FMS-like tyrosine kinase 3 (FLT3) is a receptor tyrosine kinase that is expressed in both normal and malignant lympho-hematopoietic cells and is important for immune response and stem cell proliferation. The characteristic domain organization of these receptors includes an extracellular module, a transmembrane (TM) helix, and an intracellular module that consists of a juxtamembrane (JM) segment, a kinase domain with a kinase insert region, and a C-terminal tail. The deregulated activation of FLT3 due to mutation or overexpression is linked to the progression of acute myeloid leukemia (AML) and is associated with poor prognosis. Chemical optimization of these compounds led to the discovery of quizartinib or AC220, which exhibits both selectivity for and potency against FLT3.

Here, we determined the co-crystal structure of FLT3 bound to quizartinib. FLT3 adopts an “Abl-like” inactive conformation with quizartinib bound. The DFG motif adopts a “DFG-out” conformation, the activation loop is folded back onto the kinase domain to mimic peptide substrate binding, and Glu 661 on the αC helix forms a salt bridge with Lys 644 in the active site. One favorable interaction observed in the quizartinib-FLT3 co-crystal structure, in contrast to the top-ranked docking pose, is between the tert-butyl substituent on the isoxazole ring of quizartinib and a hydrophobic pocket on FLT3. The pocket includes Met 664 and Met 665 on the αC helix, Ile 674 in the N lobe, Leu 802 in the C lobe, and Ile 827, which is immediately N terminal to the DFG motif. The carbonyl group of the urea forms hydrogen bond interactions with the backbone nitrogen of Cys 828. Further, the nitrogens in the urea moiety form hydrogen bond interactions with Glu 661 in the αC helix. The central para-substituted phenyl ring on quizartinib makes key interactions in the kinase active site of FLT3. This ring is sandwiched between the gatekeeper residue, Phe 691, and the phenylalanine residue in the DFG motif, Phe 830. The juxtamembrane segment, however, is not observed in our structure, and would not be compatible with quizartinib in the active site of FLT3.

>[2x]DLKWEFPRENLEFGKVLGSGAFGKVMNATAYGISKTGVSIQVAVKMLKEKADSSEREALMSELKMMTQLGSHENIVNLLGACTLSGPIYLIFEYCCYGDLLNYLRSKREKFSEDEIEYENQKRLEEEEDLNVLTFEDLLCFAYQVAKGMEFLEFKSCVHRDLAARNVLVTHGKVVKICDFGLARDIMSDSNYVVRGNARLPVKWMAPESLFEGIYTIKSDVWSYGILLWEIFSLGVNPYPGIPVDANFYKLIQNGFKMDQPFYATEEIYIIMQSCWAFDSRKRPSFPNLTSFLGCQL> ERAGPVTWVMMIACVVVFIAMQILGDQEVML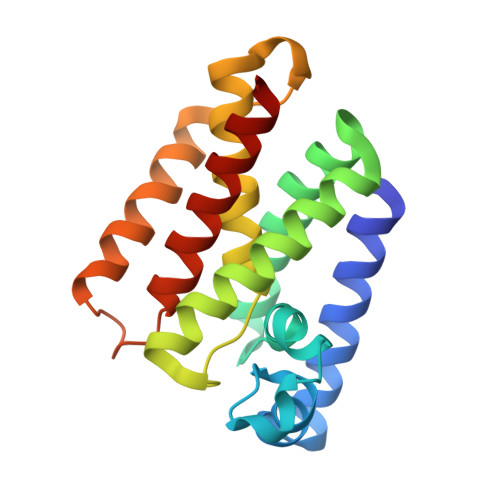WLAWPFDPTLKFEFWRYFTHALMHFSLMHILFNLLWWWYLGGAVEKRLGSGKLIVITLISALLSGYVQQKFSGPWFGGLSGVVYALMGYVWLRGERDPQSGIYLQRGLIIFALIWIVAGWFDLFGMSMANGAHIAGLAVGLAMAFVDSL> AMGAAELRFCNQTIKELMSKKHYNYNFPFL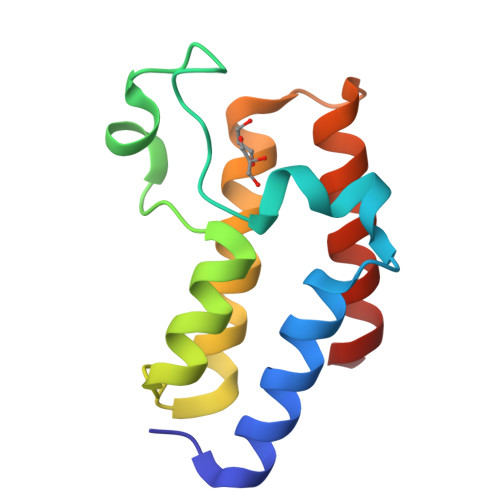APVDTVALNIPNYNEIVKQPMDLGTIQSKLANNEYENADDFEKDVRLVFKNCYLFNPEGTDVNMMGHRLEAVFDKKWAN>[5x]EAEAADRADILYNIRQTSRPDVIPTQRDRPVAVSVSLKFINIL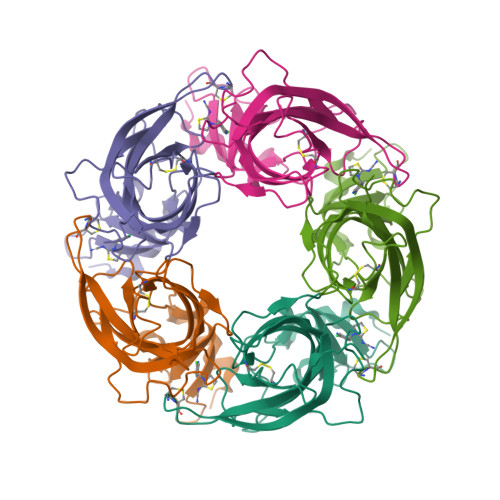EVNEITNEVDVVFWQQTTWSDRTLAWDSSHSPDQVSVPISSLWVPDLAAYNAISKPEVLTPQLARVVSDGEVLYMPSIRQRFSCDVSGVDTESGATCRIKIGSWTHHSREISVDPTTENSDDSEYFSQYSRFEILDVTQKKNSVTYSCCPEAYEDVEVSLNFRKKGRSEIL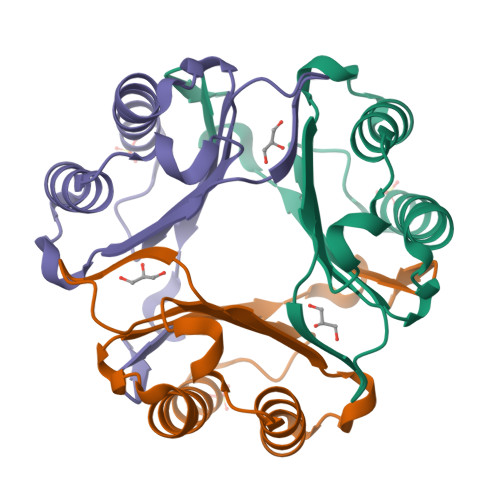>[8x]PMFIVNTNVPRASVPDGFLSELTQQLAQATGKPPQAIAVHVVPDQLMAFGGSSEPCALCSLHSIGKIGGAQNRSYSKLLCGLLAERLRISPDRVYINYYDMNAANVGWNNSTFA>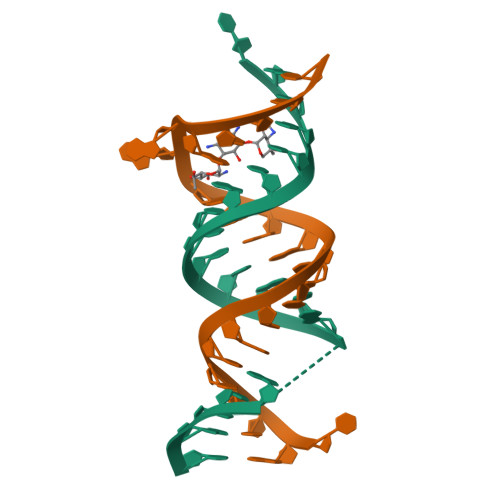[2x]UGCGUCGCUCCGGAAAAGUCGC>CSSLSIRTTDDKSLFARTMDFTMEPDSKVIIVPRNYGIRLLEKENVVINNSYAFVGMGSTDITSPVLYDGVNEKGLMGAMLYYATFATYADEPKKGTRGINPVYVISQVLGNCVTVDDVIEKLTSYTLLNEANIILGFAPPLHYTFTDASGESIVIEPDKTGITIHRKTIGVMTASPGYEWHQTNLRAYIGVTPNPPQDIMMGDLDLTPFGQGAGGLGLPGDFTPSARFLRVAYWKKYTEKAKNETEGVTNLFHILSSVNIPKGV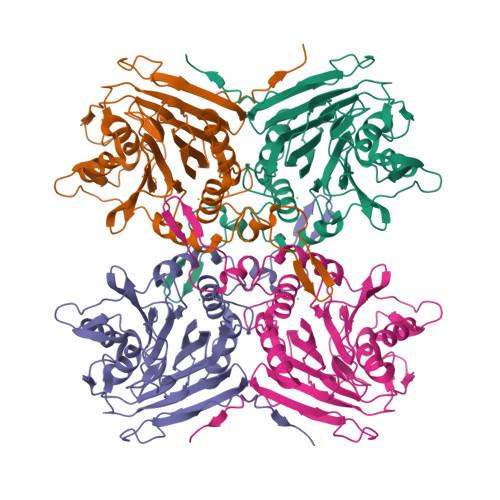VLTNEGKTDYTIYTSAMCAQSKNYYFKLYDNSRISAVSLMAENLNSQDLITFEWDRKQDIKQLNQVNVMS[8x]> LQPFKAGSVGSG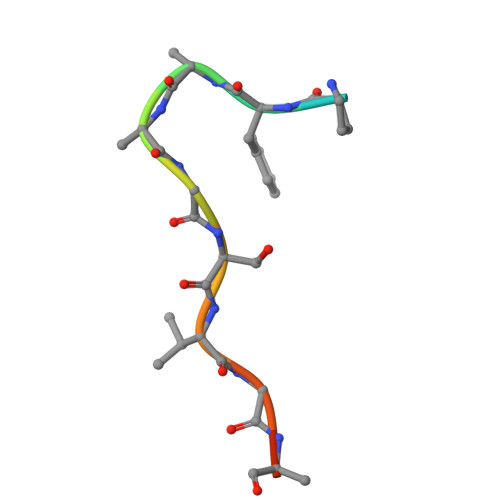S>[4x]MSLSNNTINIALIGYGFVGKTFHAPLIRSVPGLNLAFVASRDEEKVKRDLPDVTVIASPEAAVQHPDVDLVVIASPNATHAPLARLALNAGKHVVVDKPFTLDMQEARELIALAE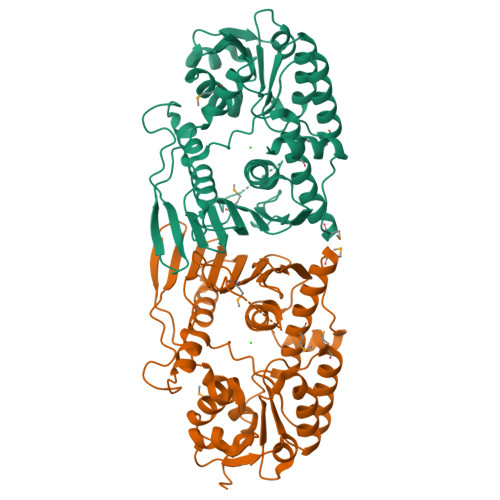EKQRLLSVFHNRRWDSDYLGIRQVIEQGTLGAVKHFESHFDRFRPEVRVRWREQNVPGSGLWFDLGPHLIDQALQLFGLPQSVQGNIATLRDGAEINDWAHVVLNYPAHKVILHCSMLVAGGSSRFTVHGDKGSVIKARADQQESQLLAGVVPGSADWGQDDDPLVIYDASLQAHAQATPQGDQRQYYMLIRDALKGQIANPVPPVEALAVMAVLEAAVRSAESGMVQTLDLSDDERNTLREGHHHHHH>[4x]KANRQREPGLGFSFEFTEQQKEFQATARKFAREEIIPVAAEYDKTGEYPVPLIRRAWELGLMNTHIPENCGGLGLGTFDACLISEELAYGCTGVQTAIEGNSLGQMPIIIAGNDQQKKKYLGRMTEEPLMCAYCVTEPGAGSDVAGIKTKAEKKGDEYIINGQKMWITNGGKANWYFLLARSDPDPKAPANKAFTGFIVEADTPGIQIGRKELNMGQRCSDTRGIVFEDVKVPKENVLIGDGAGFKVAMGAFDKTRPVVAAGAVGLAQRALDEATKYALERKTFGKLLVEHQAISFMLAEMAMKVELARMSYQRAAWEVDSGRRNTYYASIAKAFAGDIANQLATDAVQILGGNGFNTEYPVEKLMRDAKIYQIYEGTSQIQRLIVAREHIDKYKN;> MFRAAAPGQLRRAASLLRFQSTLVIAEHANDSLAPITLNTI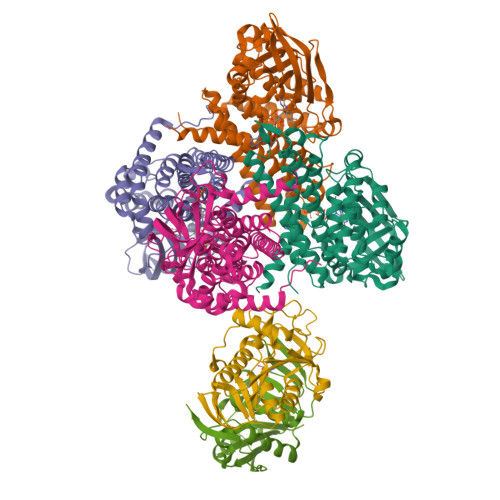TAATRLGGEVSCLVAGTKCDKVAQDLCKVAGIAKVLVAQHDVYKGLLPEELTPLILATQKQFNYTHICAGASAFGKNLLPRVAAKLEVAPISDIIAIKSPDTFVRTIYAGNALCTVKCDEKVKVFSVRGTSFDAAATSGGSASSEKASSTSPVEISEWLDQKLTKSDRPELTGAKVVVSGGRGLKSGENFKLLYDLADQLHAAVGASRAAVDAGFVPNDMQVGQTGKIVAPELYIAVGISGAIQHLAGMKDSKTIVAINKDPEAPIFQVADYGIVADLFKVVPEMTEILKKK;> MAELRVLVAVKRVIDYAVKIRVKPDRTGVVTDGVKHSMNPFCEIAVEEAVRLKEKKLVKEVIAVSCGPAQCQETIRTALAMGADRGIHVEVPPAEAERLGPLQVARVLAKLAEKEKVDLVLLGKQAIDDDCNQTGQMTAGFLDWPQGTFASQVTLEGDKLKVEREIDGGLETLRLKLPAVVTADLRLNEPRYATLPNIMKAKKKKIEVIKPGDLGVDLTSKLSVISVEDPPQRTAGVKVETTEDLVAKLKEIGRI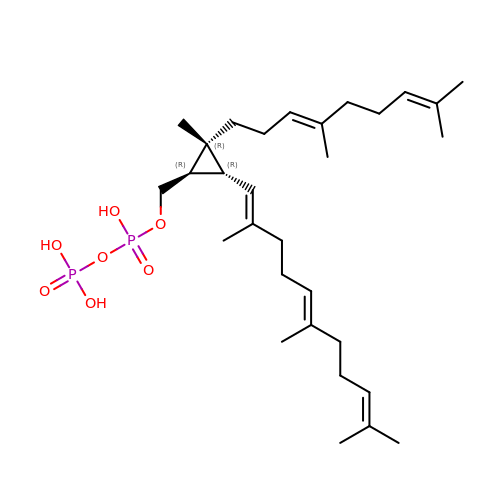{(1R,2R,3R)-2-[(3E)-4,8-dimethylnona-3,7-dien-1-yl]-2-methyl-3-[(1E,5E)-2,6,10-trimethylundeca-1,5,9-trien-1-yl]cyclopropyl}methyl trihydrogen diphosphate | C30 H52 O7 P2 | ATZKAUGGNMSCCY-VVFNRDJMSA-N> HHMLLWRRCRAWLEIRRLDKELAQSSGLPLELPQIVPNAWNEVVWRLPVPNHPDAFMTASNAAQSDFIVYVNGLAFYRAWLALGVEDSQACPLKQDMPKDRKYPSSAAHFAVGIDSPVPLADVSPTMILGHFAVCFT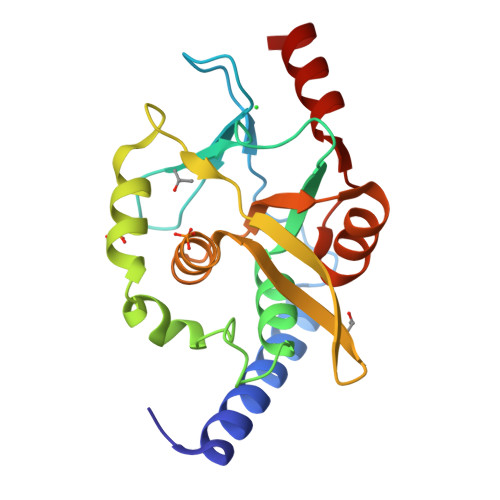DGMTRSMWLLAHEVAVFPVLSRDEASAVMLAEHVGVAAPIQVSKLREQCRKIL> MTSEQTGEPAEDTSGVIKMAVKFDRRAYPAQITPKMCLLEWCRREKLAQPVYETVQRPLDRLFSSIVTVAEQKYQSTLWDKSKKLAEQAAAIVCLRSQGLPEGRLGEESPSLHKHHHHHH

However, this belief has recently been challenged by the discovery of a dsRBD serving as a major tRNA binding module for human dihydrouridine synthase 2 (hDus2), a flavoenzyme that catalyzes synthesis of dihydrouridine within the complex elbow structure of tRNA. Dus2 is found in all eukaryotes and catalyzes formation of dihydrouridine 20 in tRNA. However, in stark contrast, we showed that, despite the presence of a HD domain, hDus2 and by inference from the sequences probably all animal ones instead use a novel extended dsRBD version flanked by a peculiar N-terminal extension (NTE) and C-terminal extension (CTE) to provide the major binding sites for tRNA substrate. By solving the crystal structure of this dsRBD in complex with a dsRNA together with extensive characterizations of its interaction with tRNA using mutagenesis, NMR and SAXS, we establish that while hDus2 dsRBD retains a conventional dsRNA recognition capability, the presence of an N-terminal extension appended to the canonical domain provides additional residues for binding tRNA in a structure-specific mode of action.

To investigate how this novel extended dsRBD recognizes a dsRNA molecule, we crystallized hDus2′s dsRBD (construct T339-K451 of human Dus2) in complex with an eleven palindromic oligo-ribonucleotide and solved the whole structure. The designed dsRNA, which harbors two overhangs at the 3′-extremities, self-assembles into a pseudo A-helix. Overall, there are no major structural changes detected between free and bound dsRBD, except for a notable modification in the twist of the C-terminal region of strand β1 induced by dsRNA that consequently alters loop β1–β2 conformation. Recognition of dsRNA is essentially achieved via three major canonical regions namely helix-α1, helix-α2 and the C-terminal part of the β1–β2 loop. Three residues of helix-α1 (T369, E376, R379) interact with ribose 2′-OH groups in dsRNA’s minor groove while K371 of helix-α1 together with K419, K420 and Q424 located in the N-terminal extremity of helix α2 recognize exclusively the phosphodiester backbone of the major groove. Remarkably, the C-terminal part of the β1–β2 loop binds to the mG+1 minor groove via R397, which makes hydrogen bonds with both the ribose and nucleobase C10. Note that animal Dus2 dsRBDs have a shorter β1–β2 loop, with 2–3 residues less than the one of archetypal dsRBDs, preventing the canonical mode of RNA recognition via this loop, and likely explaining the peculiar contacts observed for this region in the dsRBD-RNA structure (see also the discussion). Although the majority of dsRNA recognition is ensured by interactions involving the canonical fold, our structure reveals that there is a residue Q367 located in the NTE, more precisely between the 310 helix and the beginning of helix-α1 that also participates to dsRNA recognition. Q367 interacts with C8, A’3 and G’2 in proximity to helix-α1 binding site further extending the interaction surface with the minor groove.The LytR-CpsA-Psr (LCP) (LytR - autolysin regulator; CpsA–capsule-associated protein A and Psr–penicillin-binding protein regulator) is a family of enzymes responsible for the last step of the assembly of WTA and other cell wall glycopolymers. LytR and other members of the LCP family have been described as pyrophosphatases. They cleave the pyrophosphate bond in glycopolymers precursors. In this work, we studied the LytR protein from the Gram-positive bacterium Streptococcus dysgalactiae subsp. dysgalactiae (SDSD), a known animal pathogen and one of the leading causes of bovine mastitis and fish streptococcosis.

In this study, the structure of the LCP domain of LytR protein from S. dysgalactiae subsp. dysgalactiae was determined at 2.80 Å, confirming that despite low sequence homology with other LCP-family members, the overall structure is highly conserved. Analysis of the electron density maps suggests the presence of three sulphate ions at the surface of the protein. No electron density was observed at the active site that could correspond to bound substrates. The regions S48-Q56, G70-Q77, and N335-S342 are highly disordered, with no interpretable electron density in the 2Fo-Fc map. The structure is composed of 8 α-helices alternated with 12 β-sheets in a 3-layer (αβα) sandwich architecture. The characteristic central six-stranded β-sheet is sandwiched between the α-helices and the double-stranded antiparallel β-sheets (β4-β5, β7-β8 and β11-β12). LytR LCP domain contains a long and narrow pocket located between the central β-strand and the α-helices 3 to 7, near the N-terminus. The presence of this pocket is extremely conserved in the LCP family of proteins corresponding to the binding site of the undecaprenyl units - the hydrophobic section - of the physiological substrates. The binding site of LCP proteins is composed of conserved positive and negatively charged residues: two aspartates (D68 and D83 for SDSD LytR) coordinate the Mg2+ cofactor and are present in all members of the family identified so far, except for just two cases. The positive charges come from four conserved arginines (R154, R210, R212 and R222 for SDSD LytR) that are expected to interact with the pyrophosphate group present in the native substrates.

> MSKKSDAIKQTKSFSILLMGVDTGSSERTSQWEGNSDSMILVTVNPETKKTTMTSLERDILITLSGPKNNDMNGAEAKLNAAYAAGGAQMAIMTVQDLLNITIDNYVQINMQGLIDLVDAVGGITVTNEFDFPISIADNEPEYQATVAPGTHKVNGEQALVYARMRYDDPEGDYGRQKRQREVIQKVLKKILALDSISSYRKILSAVSGNMQTNIEISSNTIPGLLGYRDALKTIKTYQLKGEDATLSDGGSYQIVTSDHLLETQNRIRGELGLRKVTQLKTSATVYENLYGSRKSALEHHHHHH> RTEDLPKAVVFLEPQWYRVLEKDSVTLKCQGAYSPEDNSTQWFHNESLISSQASSYFIDAATVDDSGEY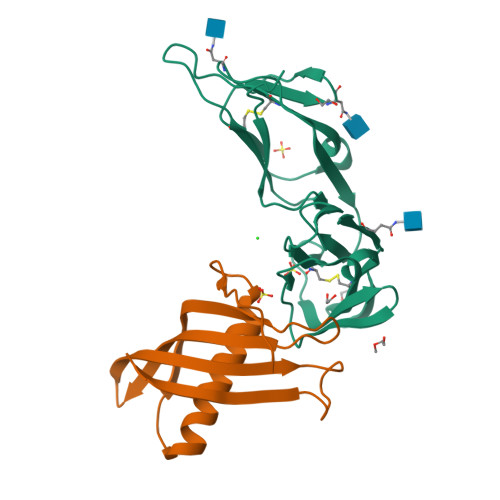RCQTNLSTLSDPVQLEVHIGWLLLQAPRWVFKEEDPIHLRCHSWKNTALHKVTYLQNGKGRKYFHHNSDFYIPKATLKDSGSYFCRGLVGSKNVSSETVNITITQG;> AQLHSTVRAVPGNENSLEIEELARFAVDEHNKKENALLEFVRVVKAKEQYEDEHWFPGTMYYLTLEAKDGGKKKLYEAKVWVKNTAAPPSHMNFKELQEFKPVGDAAAAHHHHHH>SSPATSPQSTPTLVSALETIEPEVLYAGYDSSVPDSTWRIMTTLNMLGGRQVIAAVKWAKAIPGFRNLHLDDQMTLLQYSWMYLMAFALGWRSYRQSSANLLCFAPDLIINEQRMTLPDMYDQCKHMLYVSSELHRLQVSYEEYLCMKTLLLLSSVPKDGLKSQALFDAIRMTYIKELGKAIVKREGNSSQNSQRFYQLTKLLDSMHEVVENLLNYCFQTFLDKTM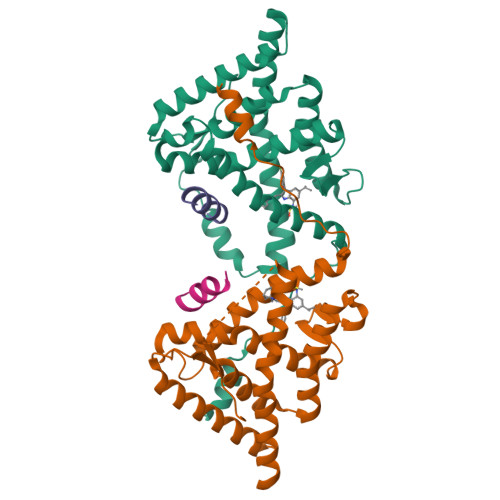SIEFPEMLAEIITNQIPKYSNGNIKKLLFHQK[2x];>[2x]NLGLEDIIRKALMGS>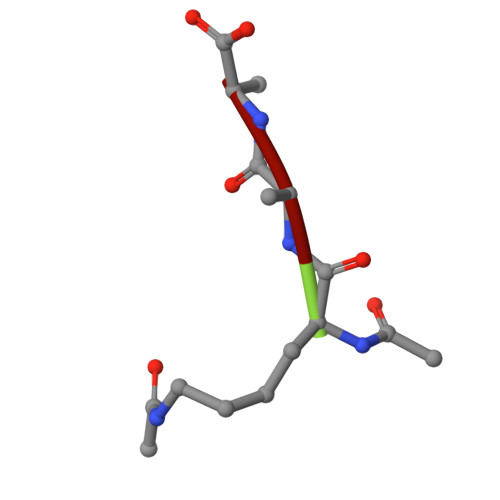 KAA> MPIRQMKDSSETHLVIKTQPLKHHNPKTVQNGKIPPPSPSPVTVTTPATVTQSQASSPSPPSKNRSRRRNRGGRKSDQGDVCMRPSSRPRKPPPPSQTTSSAVSVATAGEIVAVNHQMQMGVRKNSNFAPRPGFGTLGTKCIVKANHFLADLPTKDLNQYDVTITPEVSSKSVNRAIIAELVRLYKESDLGRRLPAYDGRKSLYTAGELPFTWKEFSVKIVDEDDGIINGPKRERSYKVAIKFVARANMHHLGEFLAGKRADCPQEAVQILDIVLRELSVKRFCPVGRSFFSPDIKTPQRLGEGLESWCGFYQSIRPTQMGLSLNIDMASAAFIEPLPVIEFVAQLLGKDVLSKPLSDSDRVKIKKGLRGVKVEVTHRANVRRKYRVAGLTTQPTRELMFPVDENCTMKSVIEYFQEMYGFTIQHTHLPCLQVGNQKKASYLPMEACKIVEGQRYTKRLNEKQITALLKVTCQRPRDRENDILRTVQHNAYDQDPYAKEFGMNISEKLASVEARILPAPWLKYHENGKEKDCLPQVGQWNMMNKKMINGMTVSRWACVNFSRSVQENVARGFCNELGQMCEVSGMEFNPEPVIPIYSARPDQVEKALKHVYHTSMNKTKGKELELLLAILPDNNGSLYGDLKRICETELGLISQCCLTKHVFKISKQYLANVSLKINVKMGGRNTVLVDAISCRIPLVSDIPTIIFGADVTHPENGEESSPSIAAVVASQDWPEVTKYAGLVCAQAHRQELIQDLYKTWQDPVRGTVSGGMIRDLLISFRKATGQKPLRIIFYRAGVSEGQFYQVLLYELDAIRKACASLEPNYQPPVTFIVVQKRHHTRLFANNHRDKNSTDRSGNILPGTVVDTKICHPTEFDFYLCSHAGIQGTSRPAHYHVLWDENNFTADGIQSLTNNLCYTYARCTRSVSIVPPAYYAHLAAFRARFYLEPEIMQDNGSPGKKNTKTTTVGDVGVKPLPALKENVKRVMFYC

The loading of sRNA duplexes into the proper ARGONAUTE (AGO) protein is a key step to forming a functional silencing complex. AGO proteins are composed of N-terminal (N), Linker-1 (L1), PAZ, Linker-2 (L2), MID and PIWI domains to form a bilobed structure with a cleft in the center to retain the sRNA. Arabidopsis thaliana expresses two AGO proteins, AtAGO7 and AtAGO10, that display remarkably exclusive sRNA loading preferences, with each largely dedicated to one or two specific sRNAs. Thus, a major, albeit noncanonical function of AtAGO10 is to bind miR165/166 and promote its degradation, thereby limiting the loading of miR165/166 into AtAGO1 and elevating the expression levels of miR165/166 targeted genes that are important to maintaining the stemness of the SAM.

A loop in the AtAGO10 central cleft is essential for recognizing specific mismatches opposite the guide strand 3′ region in miR166/165 duplexes. Replacing this loop with the equivalent loop from Homo sapiens AGO2 (HsAGO2) changes AtAGO10 miRNA loading behavior such that 3′ region mismatches are ignored and mismatches opposite the guide 5′ end instead drive loading, as in HsAGO2. Mismatches at positions 12 and 13 of the miR166 diplex are important for miR166 recognition by AtAGO10 in vivo. Examining the AtAGO10 structure, we identified five loops in the central cleft (first loop: residues 287–288, second loop: residues 714–720, third loop: residues 747–751, fourth loop: residues 796–800, fifth loop: residues 835–840) that are located near miRNA duplex base pairs involving guide strand nucleotides 12 and 13. Thus, we hypothesized that one or more of these loops may participate in the recognition of the 12–13 mismatches. Aligning the primary sequences of HsAGO2 and AtAGO10 revealed that the second central loop is divergent, while the other four loops are highly conserved. Thus, we suspected that the second loop might be responsible for the difference in duplex selectivity between AtAGO10 and HsAGO2. We tested this hypothesis by replacing the second central loop in AtAGO10 (residues 714–720) with the sequence of the corresponding loop in HsAGO2, and expressing and purifying the resulting AtAGO10 mutant protein (AtAGO10-714-720-Hs). Thus, the second central loop plays an essential role in establishing the specialized duplex selectivity of AtAGO10, possibly through direct recognition of the mismatched 12–13 region of miR166/165 duplexes. We therefore reason that, in addition to opening the AtAGO10 central cleft to enable duplex loading, the chaperon system also positions the central loop for recognition of the miRNA duplex near the guide 3′ region.>MQQGQMAYDRAITVFSPDGRLFQVEYAREAVKKGSTALGMKFANGVLLISDKKVRSRLIEQNSIEKIQLIDDYVAAVTSGYVADARVLVDFARISAQQEKVTYGSLVNIENLVKRVADQMQQYTQYGGVRPYGVSLIFAGIDQIGPRLFDCDPAGTINEYKATAIGSGKDAVVSFLEREYKENLPEKEAVTLGIKALKSSLEEGEELKAPEIASITVGNKYRIYDQEEVKKFL[14x];>MNQTLETGTTTVGITLKDAVIMATERRV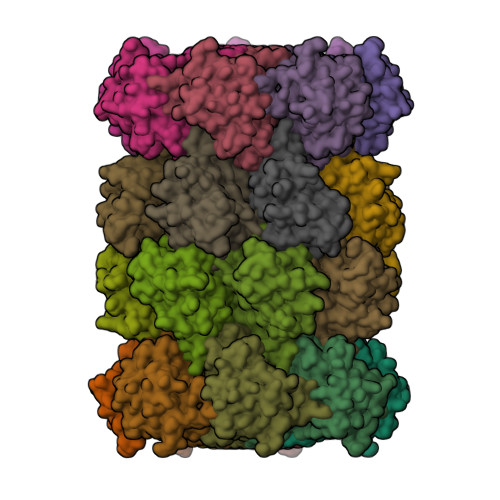TMENFIMHKNGKKLFQIDTYTGMTIAGLVGDAQVLVRYMKAELELYRLQRRVNMPIEAVATLLSNMLNQVKYMPYMVQLLVGGIDTAPHVFSIDAAGGSVEDIYASTGSGSPFVYGVLESQYSEKMTVDEGVDLVIRAISAAKQRDSASGGMIDVAVITRKDGYVQLPTDQIESRIRKLGLIL[14x]3-(4-chlorophenyl)-5,6-dihydroimidazo[2,1-b][1,3]thiazole | C11 H9 Cl N2 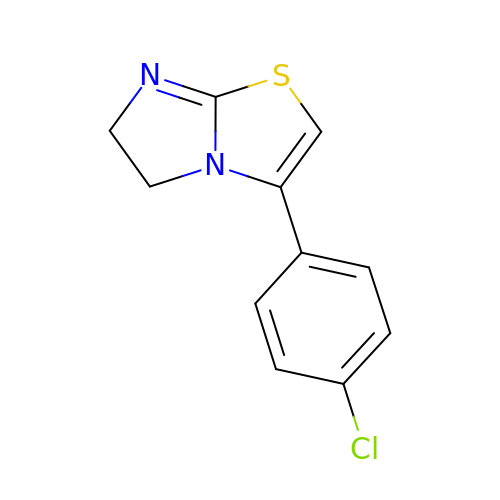S | DFKOPKKSCIVOAK-UHFFFAOYSA-N>[2x]LDVPCKVVITAPEGEDPHPRFGKVEMSHA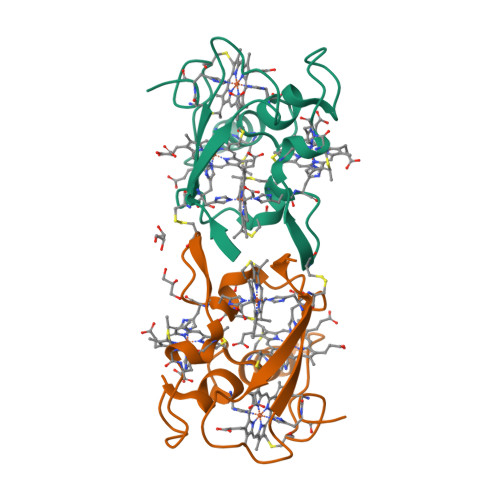KHRNVSCVSCHHMFDGCGDFQKCADCHIDRDDRSYERGFYKAWHSESEISCRGCHKAMKAKNEQTGPIGCLQGCHEAAQK1-METHYL ETHYL 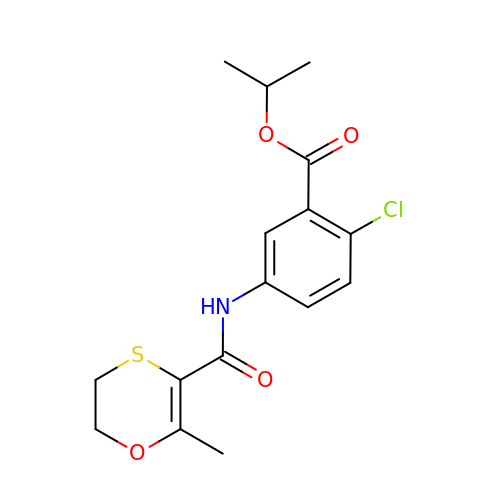1-CHLORO-5-[[(5,6DIHYDRO-2-METHYL-1,4-OXATHIIN-3-YL)CARBONYL]AMINO]BENZOATE | C16 H18 Cl N O4 S | FMQGUMRNTBJHEA-UHFFFAOYSA-N>[2x]NAKGNYCKRTPLYIDFKEIGWDSWIIAPPGYEAYECRGVCNYPLAEHLTPTKHAIIQALVHLKNSQKASKACCVPTKLEPISILYLDKGVVTYKFKYEGMAVSECGCR;>SPIMNLEQS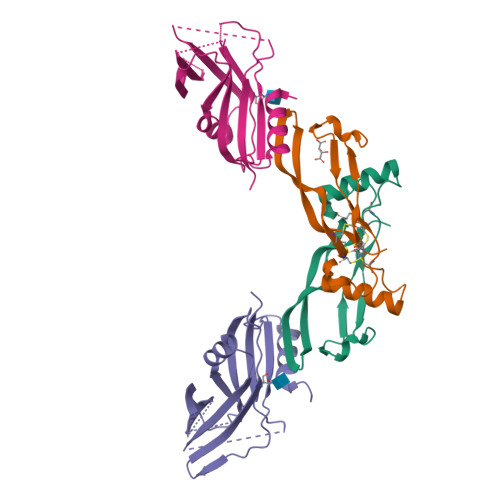PLEEDMSLFGDVFSEQDGVDFNTLLQSMKDEFLKTLNLSDIPTQDSAKVDPPEYMLELYNKFATDRTSMPSANIIRSFKNEDLFSQPVSFNGLRKYPLLFNVSIPHHEEVIMAELRLYTLVQRDRMIYDGVDRKITIFEVLESKGDNEGERNMLVLVSGEIYGTNSEWETFDVTDAIRRWQKSGSSTHQLEVHIESKHDEAEDASSGRLEIDTSAQNKHNPLLIVFSDDQSSDKERKEELNEMISHEQLPELDNLGLDSFSSGPGEEALLQMRSNIIYDSTARIRR[2x]>NLIKQLQERGLVAQVTDEEALAERLAQGPIALYCGFDPTADSLHLGHLVPLLCLKRFQQAGHKPVALVGGATGLIGDPSFKAAERKLNTEETVQEWVDKIRKQVAPFLDFDCGENSAIAANNYDWFGNMNVLTFLRDIGKHFSVNQMINKEAVKQRLNREDQGISFTEFSYNLLQGYDFACLNKQYGVVLQIGGSDQWGNITSGIDLTRRLHQNQVFGLTVPLITKADGTKFGKTEGGAVWLDPKKTSPYKFYQFWINTADADVYRFLKFF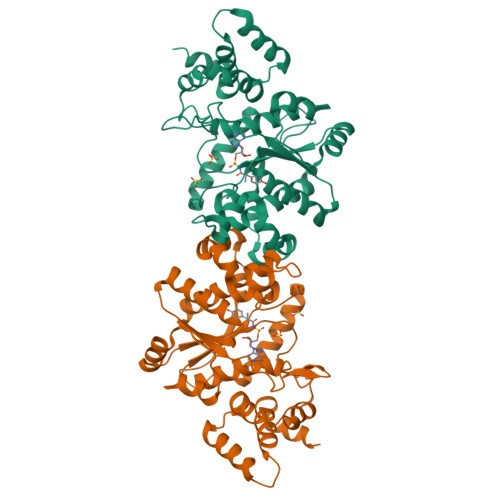TFMSIEEINALEEEDKNSGKAPRAQYVLAEQVTRLVHGEEGLQAAKR[2x]> MKEFYLTVEQIGDSIFERYIDSNGRERTREVEYKPSLFAHCPESQATKYFDIYGKPCTRKLFANMRDASQWIKRMEDIGLEALGMDDFKLAYLSDTYNYEIKYDHTKIRVANFDIEVTSPDGFPEPSQAKHPIDAITHYDSIDDRFYVFDLLNSPYGNVEEWSIEIAAKLQEQGGDEVPSEIIDKIIYMPFDNEKELLMEYLNFWQQKTPVILTGWNVESFDIPYVYNRIKNIFGESTAKRLSPHRKTRVKVIENMYGSREIITLFGISVLDYIDLYKKFSFTNQPSYSLDYISEFELNVGKLKYDGPISKLRESNHQRYISYNIIDVYRVLQIDAKRQFINLSLDMGYYAKIQIQSVFSPIKTWDAIIFNSLKEQNKVIPQGRSHPVQPYPGAFVKEPIPNRYKYVMSFDLTSLYPSIIRQVNISPETIAGTFKVAPLHDYINAVAERPSDVYSCSPNGMMYYKDRDGVVPTEITKVFNQRKEHKGYMLAAQRNGEIIKEALHNPNLSVDEPLDVDYRFDFSDEIKEKIKKLSAKSLNEMLFRAQRTEVAGMTAQINRKALINGLAGALGNVWFRYYDLRNATAITTFGQMALQWIERKVNEYLNEVCGTEGEAFVLYG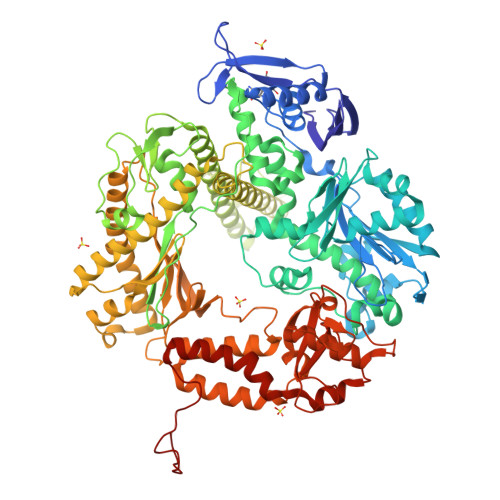DTDSIYVSADKIIDKVGESKFRDTNHWVDFLDKFARERMEPAIDRGFREMCEYMNNKQHLMFMDREAIAGPPLGSKGIGGFWTGKKRYALNVWDMEGTRYAEPKLKIMGLETQKSSTPKAVQKALKECIRRMLQEGEESLQEYFKEFEKEFRQLNYISIASVSSANNIAKYDVGGFPGPKCPFHIRGILTYNRAIKGNIDAPQVVEGEKVYVLPLREGNPFGDKCIAWPSGTEITDLIKDDVLHWMDYTVLLEKTFIKPLEGFTSAAKLDYEKKASLFDMFDFHHHHHH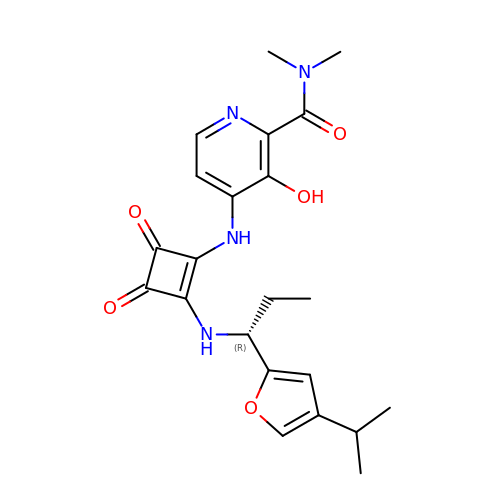4-[[3,4-bis(oxidanylidene)-2-[[(1~{R})-1-(4-propan-2-ylfuran-2-yl)propyl]amino]cyclobuten-1-yl]amino]-~{N},~{N}-dimethyl-3-oxidanyl-pyridine-2-carboxamide | C22 H26 N4 O5 | JSZQMZJVSCVDMA-CYBMUJFWSA-N>MPSNNRYDVTEWPAGNPAKDIGEVINSIIADIKARQGAADVDDGGKPGAVIYLPPGDYHLRTQVLIDISFLRIEGSGHGFTSSSIRFNVPEEEWPDLHELWPGGSRVIVDLPAGGAGDSAAGAAFLVAREGSPRISSVEFSNFCIDGLHFTADGSGRHPENTYANGKTGIHVASANDSFRVTDMGFVYLENALTIHKADALSIHHNFIAECGSCIELRGWGQASKITDNLVGAGPRGHSIYAENHGGLLVTANNVFPRGASSVHFKGVTRSSVTNNRLHAFYPGMVRLEENSSENL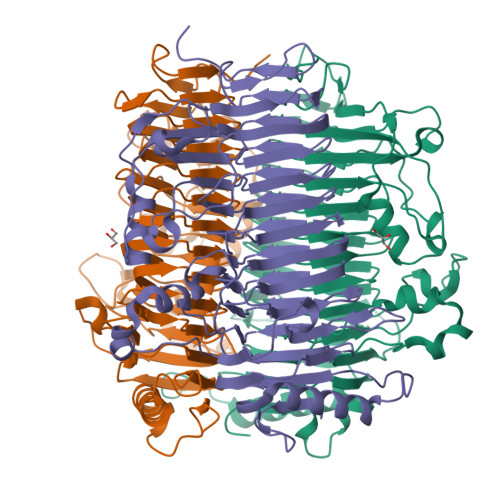VATNHFLRDHEPWTPFFGVDNGLDDLTGLLSISGNNNSVIGNHFSEVVDANEIRPEGATPVIIRLTAGTGNFVSTNHVVAMDVDAASSDSAFEAQVDALLATEAADLAVTAVLVDPGSARNTILDSGSDTQVVADRAVNAIRATPTVGF[6x]> MPVLKVMFHKDTNVATVLDASGSLSDGSVEVGTFHHPDETYPDSVT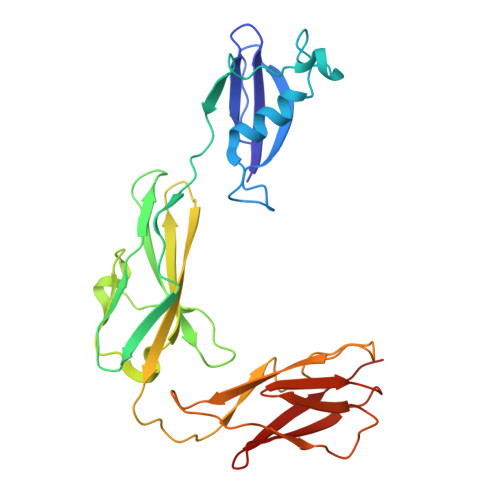IYHGVRDLLYKRSAKDPSQTASYPNNIINMQVISIDMKATPRLILGTALPRVISTIEGKDVTWHVDVAGGKAPLTYKWQFKANTVGAAFADIDSGENPTAKTATLINHAVTAESAGTYKVIVTDANGTTIESSSLLVVGVQEPPEVASIVAYPSPLALSVADDITDGKTVKFSSLPAGSLIGTLSIKTQPDSGKATAEISGNVLTVKPVAAGDTTVVVTNGTKEVTVTVNVTE> FECPGGRLTPQQRKDIVRQNNKFRSLLIHGKLKNRNGTYMPRGKNMLLLKWSCQLENSAQRWANQCVFGHSPRNQRQGIGENVYAYWSSESVEKLRNTAGTEAGKSWW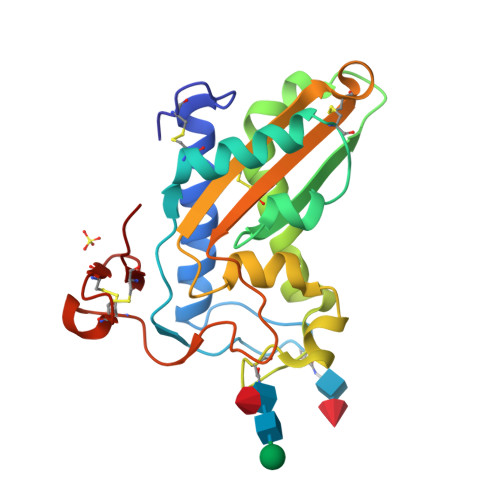SELPKLYKQNPSNNLTDDVARQGVLHFTQMAWGKTHKIGCGIATNCDGGRTLIAICHYSPAGNMLKELIYELGEPCKTDSDCNTKKCAKKSGLCRKEL> SVLQVLHIPDERLRKVAKPVEEVNAEIQRIVDDMFETMYAEEGIGLAATQVDIHQ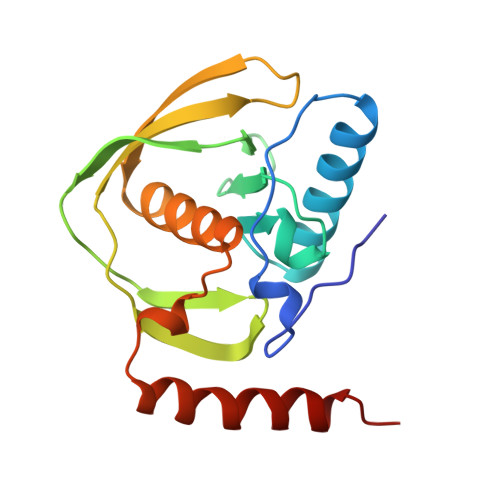RIIVIDVSENRDERLVLINPELLEKSGETGIEEGCLSIPEQRALVPRAEKVKIRALDRDGKPFELEADGLLAICIQHEMDHLVGKLFMDYLSPLKQQRIRQKVEKLDRLKARA> AQHITPVSEKKVDDKITLYKTTATSDSDKLKISQILTFNFIKDKSYDKDTLILKAAGNIYSGYTKPNPKDTISSQFYWGSKYNISINSDSNDSVNVVDYAPKN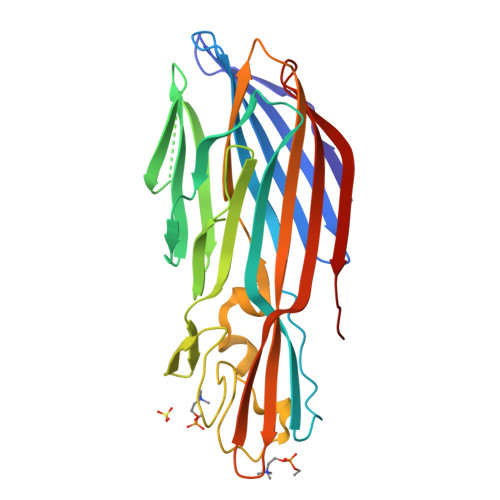QNEEFQVQQTVGYSYGGDINISNGLSGGGNGSKSFSETINYKQESYRTSLDKRTNFKKIGWDVEAHKIMNNGWGPYGRDSYHSTYGNEMFLGSRQSNLNAGQNFLEYHKMPVLSRGNFNPEFIGVLSRKQNAAKKSKITVTYQREMDRYTNFWNQLHWIGNNYKDENRATHTSIYEVDWENHTVKLIDTQSKEKNPMS>XTQEYLLKEIMKLLKEQIKLLKEQIKMLKELEKQ[5x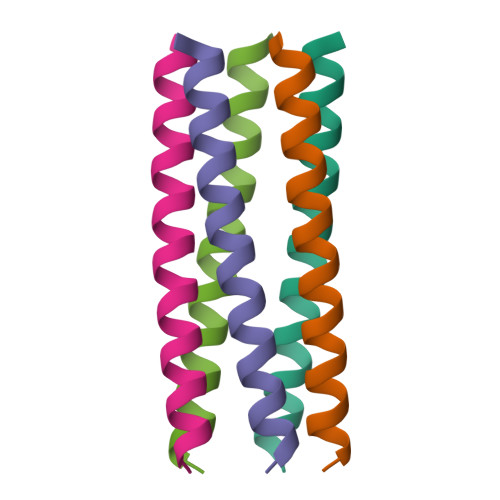]> MGPPEKDSKAILKARGLEEEQKSESTMSPSENVSRAILKDSGSEEVEQASERKMTSPENDSKSIQKDQGPEQEQTSETLQSKEEDEVTEADKDNGGDLQDYKAHVIAKFDTSVDLHYDSPEMKLLSDAFKPYQKTFQPHTIILHGRPGVGKSALARSIVLGWAQGKLFQKMSFVIFFSVREIKWTEKSSLAQLIAKECPDSWDLVTKIMSQPERLLFVIDGLDDMDSVLQHDDMTLSRDWKDEQPIYILMYSLLRKALLPQSFLIITTRNTGLEKLKSMVVSPLYILVEGLSASRRSQLVLENISNESDRIQVFHSLIENHQLFDQCQAPSVCSLVCEALQLQKKLGKRCTLPCQTLTGLYATLVFHQLTLKRPSQSALSQEEQITLVGLCMMAAEGVWTMRSVFYDDDLKNYSLKESEILALFHMNILLQVGHNSEQCYVFSHLSLQDFFAALYYVLEGLEEWNQHFCFIENQRSIMEVKRTDDTRLLGMKRFLFGLMNKDILKTLEVLFEYPVIPTVEQKLQHWVSLIAQQVNGTSPMDTLDAFYCLFESQDEEFVGGALKRFQEVWLLINQKMDLKVSSYCLKHCQNLKAIRVDIRDLLSVDNTLELCPVVTVQETQCKPLLMEWWGNFCSVLGSLRNLKELDLGDSILSQRAMKILCLELRNQSCRIQKLTFKSAEVVSGLKHLWKLLFSNQNLKYLNLGNTPMKDDDMKLACEALKHPKCSVETLRLDSCELTIIGYEMISTLLISTTRLKCLSLAKNRVGVKSMISLGNALSSSMCLLQKLILDNCGLTPASCHLLVSALFSNQNLTHLCLSNNSLGTEGVQQLCQFLRNPECALQRLILNHCNIVDDAYGFLAMRLANNTKLTHLSLTMNPVGDGAMKLLCEALKEPTCYLQELELVDCQLTQNCCEDLA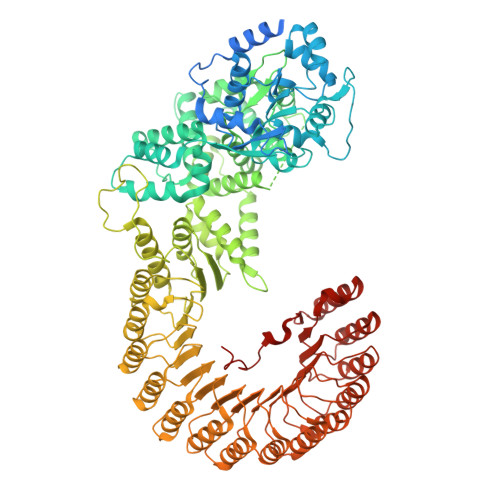CMITTTKHLKSLDLGNNALGDKGVITLCEGLKQSSSSLRRLGLGACKLTSNCCEALSLAISCNPHLNSLNLVKNDFSTSGMLKLCSAFQCPVSNLGIIGLWKQEYYARVRRQLEEVEFVKPHVVIDGDWYASDEDDRNWWKN>[2x]MNHKVHHHHHHMELGTLEGSMAGARCRTLYPFSGERHSQGLRFSAGELLTLLQVPDGGWWEGEKDDGLRGWFPASYVQLLEKPGMVPPPPGEESQTVILPPGWHSYLSPQGRRYYVNTTTNETTWERPSSSPGISASPGPHRSSLPTTVNGYHASGTPAHPPETAHMSLRKSTGDSQNLGSSSPGR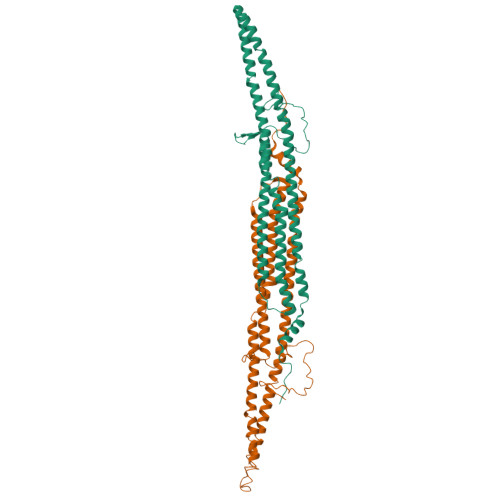KQSKENTITINCVTFPHPDTMPEQQLLKPTEWSYCDYFWADKKDPQGNGTVAGFELLLQKQLKGKQMQKEMSEFIRERIKIEEEYAKNLAKLSQNSLAAQEEGSLGEAWAQVKKSLADEAEVHLKFSAKLHSEVEKPLMNFRENFKKDMKKCDHHIADLRKQLASRYASVEKARKALTERQKDLEMKTQQLEIKLSNKTEEDIKKARRKSTQAGDDLMRCVDLYNQAQSKWFEEMVTTTLELERLEVERVEMIRQHLCQYTQLRHETDMFNQSTVEPVDQLLRKVDPAKDRELWVREHKTGNIRPVDMEI> GHMKQEELKRLYKAQAIQRQLEEVEERQRASEIQGVRLEKALRGEADSGTQDEAQLLQEWFKLVLEKNKLMRYESELLIMAQELELEDHQSRLEQKLREKMLKEESQKDE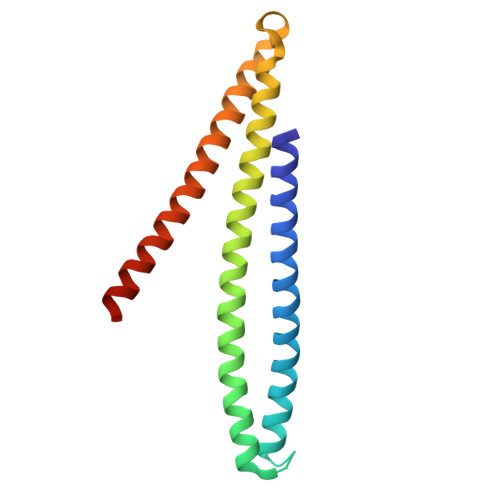KDLNEEQEVFTELMQVIEQRDKLVDSLEEQRIREKAEDQHFES>[13x]MAIDVLDVISLSLF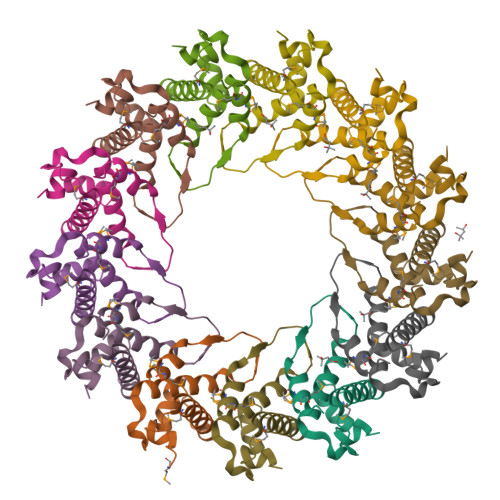KQQIEFEEDDRDELITLYAQAAFDYCMRWCDEPAWKVAADIPAAVKGAVLLVFADMFEHRTAQSEVQLYENAAAERMMFIHRNWRGKAESEEGS> MKEQLEDVLDTLTDREENVLRLRFGLDDGRTRTLEEVGKVFGVTRERIRQIEAKALRKLRHPSRSKRLKDFMD;> MKLKILDKDNATLNVFHRNKEHKTIDNVPTANLVDWYPLSNAYEYKLSRNGEYLELKRLRSTLPSSYGLDDNNQDIIRDNNHRCKIGYWYNPAVRKDNLKIIEKAKQYGLPIITEEYDANTVEQGFRDIGVIFQSLKTIVVTRYLEGKTEEELRIFNMKSEESQLNEA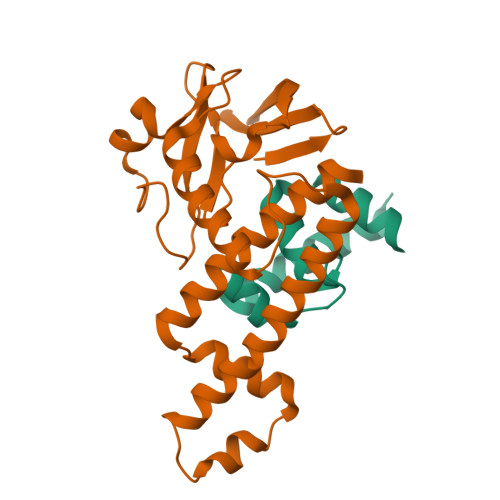LKESDFSVDLTYSDLGQIYNMLLLMKKISK>[5x]SNGLMAKRLRRELLNTYEQLGKSGLPFLDDIGKVDVKFGLSLQLLKSIEQRGMGFNSIGTFKAIVKLSWVDTILRWDPEPPFDFQKIEISPDEIWT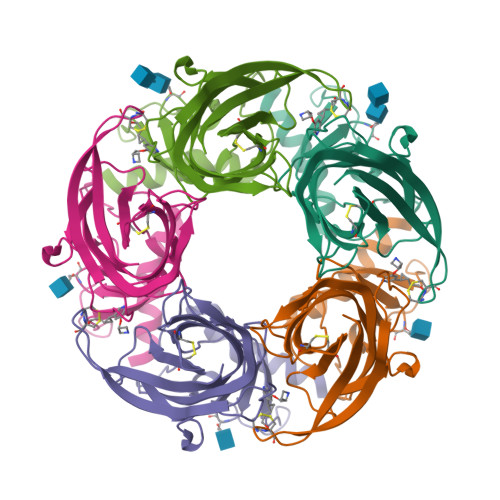PDIKLFNSVDLDMTLDRTTQAIVFSNGTVLWIPPAVLKVLCVSQDDVDSCHFQFGSWVYSVDEVDIHFMDDKAEVLLDFYQDSLEILENSAQRQEVVYPCCESAYVEMKYLLALRSENGNSTYSRDLAHHHHHH> SNAASGGRALRVLVDMDGVLADFEGGFLRKFRARFPDQPFIALEDRRGFWVSEQYGRLRPGLSEKAISIWESKN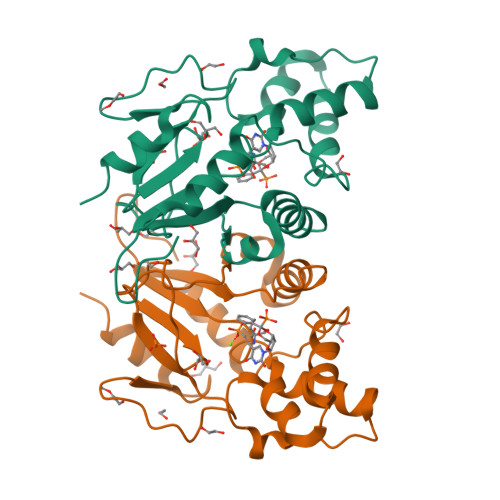FFFELEPLPGAVEAVKEMASLQNTDVFICTSPIKMFKYCPYEKYAWVEKYFGPDFLEQIVLTRDKTVVSADLLIDDRPDITGAEPTPSWEHVLFTACHNQHLQLQPPRRRLHSWADDWKAILDSKRP>[2x]GAMEDMEIAYPITCGESKAILLWKKFV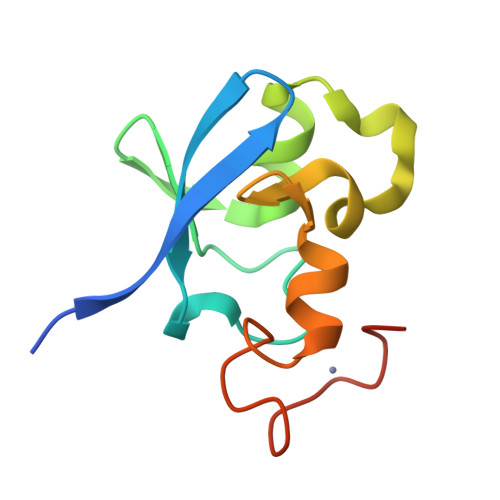CPGINVKCVKFNDQLISPKHFVHLAGKSTLKDWKRAIRLGGIMLRKMMDSGQIDFYQHDKVCSNTCRSTK> AAVEDNHLLIKAVQNEDVDLVQQLLEGGANVNFQEEEGGWTPLHNAVQMSREDIVELLLRHGADPVLRKKNGATPFLLAAIAGSVKLLKLFLSKGADVNECDFYGFTAFMEAAVYGKVKALKFLYKRGANVNLRRKTKEDQERLRKGGATALMDAAEKGHVEVLKILLDEMGADVNACDNMGRNALIHALLSSDDSDVEAITHLLLDHGADV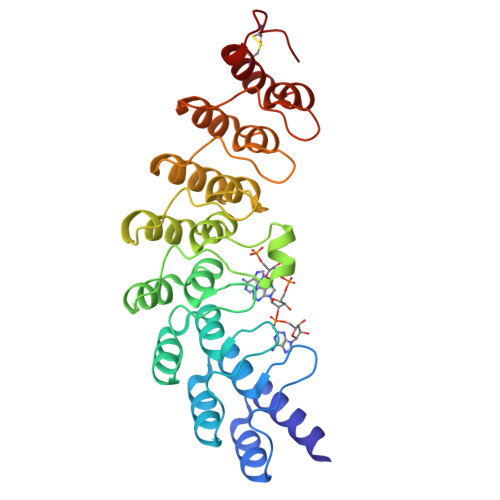NVRGERGKTPLILAVEKKHLGLVQRLLEQEHIEINDTDSDGKTALLLAVELKLKKIAELLCKRGASTDCGDLV> MAHHHHHHMTTQDELKRIAAEKA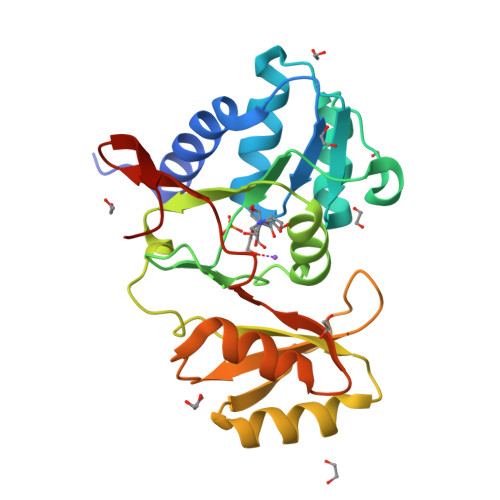VEFVPENEYIGIGTGSTINFFIEALGKSGKKIKGAVSTSKKSGELLARYDIPVVSLNEVSGLAVYIDGADEVNHALQMIKGGGGAHLNEKIVASASEKFVCIADESKYVSRLGKFPLPVEAVESARSLVSRKLLAMGGQPELRIGYTTFYGNQIVDVHGLNIDQPLTMEDEINKITGVLENGIFARDAADVLILGTEEGAKVIYPCQG N-[3-(4-methoxy-1-methyl-6-oxo-1,6-dihydropyridin-3-yl)-4-phenoxyphenyl]methanesulfonamide 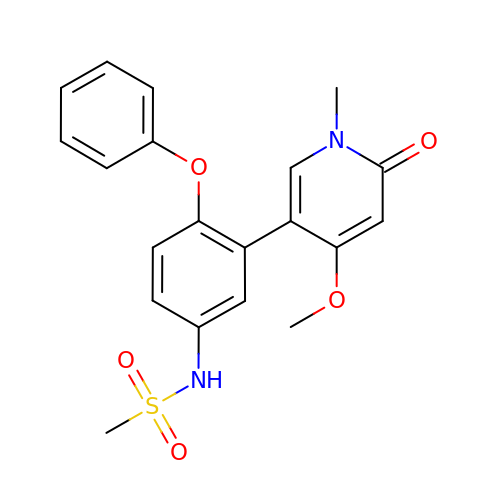| C20 H20 N2 O5 S | RHNWTJMCFPHSQX-UHFFFAOYSA-N> MGSDKIHHHHHHMKLRYLNILKEKLGREPTFVELQAFSVMWSEHCGYSHTKKYIRRLPKTGFEGNAGVVNLDDYYSVAFKIESHNHPSAIEPYNGAATGVGGIIRDVLAMGARPTAIFDSLHMSRIIDGIIEGIADYGNSIGVPTVGGELRISSLYAHNPLVNVLAAGVVRNDMLVDSKASRPGQVIVIFGGATGRDGIHGASFASEDLTGDKATKLSIQVGDPFAEKMLIEAFLEMVEEGLVEGAQDLGAGGVLSATSELVAKGNLGAIVHLDRVPLREPDMEPWEILISESQERMAVVTSPQKASRILEIARKHLLFGDVVAEVIEEPVYRVMYRNDLVMEVPVQLLANAPEEDIVEYTPGKIPEFKRVEFEEVNAREVFEQYDHM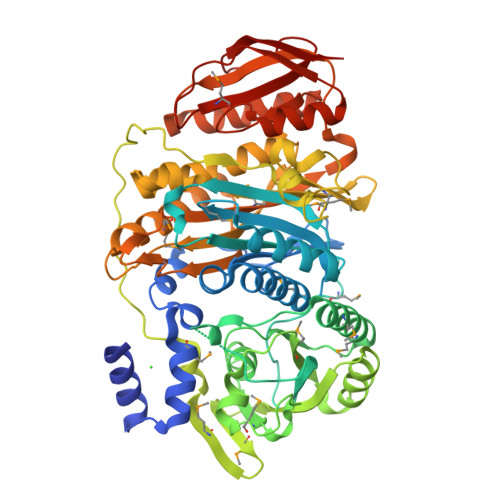VGTDTVVPPGFGAAVMRIKRDGGYSLVTHSRADLALQDTYWGTLIAVLESVRKTLSVGAEPLAITNCVNYGDPDVDPVGLSAMMTALKNACEFSGVPVASGNASLYNTYQGKPIPPTLVVGMLGKVNPQKVAKPKPSKVFAVGWNDFELEREKELWRAIRKLSEEGAFILSSSQLLTRTHVETFREYGLKIEVKLPEVRPAHQMVLVFSERTPVVDVPVKEIGTLSR> NFDAERDALNIETAIKTKGVDEVTIVNILTNRSNAQRQDIAFAYQRRTKKELASALKSALSGHLETVILGLLKTPAQYDASELKASMKGLGTDEDSLIEIICS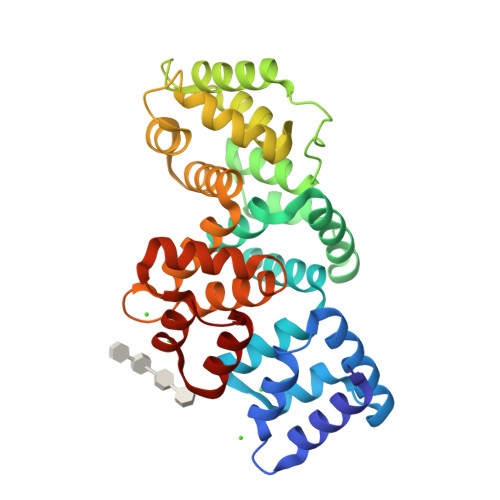RTNQELQEINRVYKEMYKTDLEKDIISDTSGDFRKLMVALAKGRRAEDGSVIDYELIDQDARDLYDAGVKRKGTDVPKWISIMTERSVPHLQKVFDRYKSYSPYDMLESIRKEVKGDLENAFLNLVQCIQNKPLYFADRLYDSMKGKGTRDKVLIRIMVSRSEVDMLKIRSEFKRKYGKSLYYYIQQDTKGDYQKALLYLCGGDD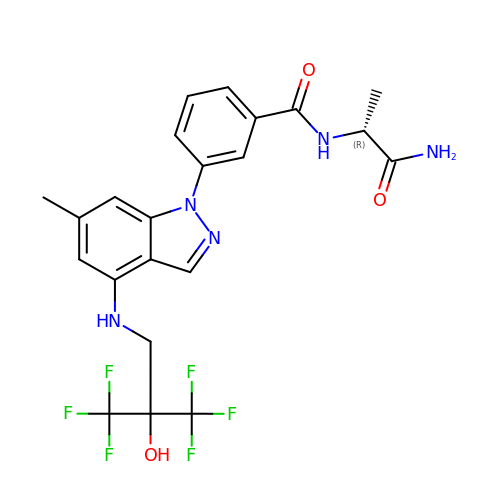N-[(1R)-2-amino-1-methyl-2-oxoethyl]-3-(6-methyl-4-{[3,3,3-trifluoro-2-hydroxy-2-(trifluoromethyl)propyl]amino}-1H-indazol-1-yl)benzamide | C22 H21 F6 N5 O3 | SDBGIXABAWIVLY-GFCCVEGCSA-N>MHHHHHHHHGGSEFSIDGGSLEVLFQGPSSPSHQIWLPPLDVPPTLDELLPPLSPSAAHGYTADGWEWRGRLHAVVGLVDRPFDQRRDPYWLDLSGGAGHVGVAGGPQTGKSTMLRTLITSLALLHTPQEVQFYCLDFGGGTLAGLAELPHVGSVATRLDADRIRRTVAEVSALLEQREQEFTERGIDSMATYRRLRATGEYAGDGFGDVFLVVDNWLTLRQDYEALEDSITQLAARGLGYGIHVVLSSNKWSEFRTSIRDLLGTKLELRLGDPYESEVDRKKAANVPENRPGRGLTRDGYHFLTALPRIDGDTSAETLTEGIATTVKTIREAWHGPTAPPVRMLPNVLPAAQLPSAAESGTRIPIGIDEDSLSPVYLDFNTDPHFLVFGDTECGKSNLLRLITAGIIERYTPQQARLIFIDYSRSLLDVATTEHQIGYAASSTAASSLVRDIKGAMEARLPPPDLTPEQLRSRSWWTGAELFLVVDDYEMVATSDNPLRPLAELLPQARDIGLHLIIARSMGGAGRALYEPIIQRIKEMASPGLVMSGNKDEGILLGNVKPHKLPQGRGYFVERRSGTRLIQTAYRES[4x];>[4x]ITYEAREEA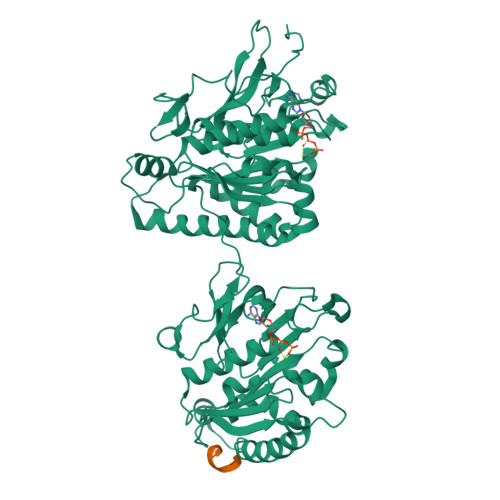AQQSVNRVQALLNG>SNASDSASKDIITMKGDTIRVSDLYKEAKQFPSQPTNTLLQNLTFDKIFTKDFGKEVTDKDVSKKVKSIKDQYGSQFSSALQQQGLTEASFTPYMRTQMLEQAAIDHEIKETQYTDANLKKAWESYHPDVTAYVVSETSKDAATKALDAAKKDDAGKASFEKTNAESKVTFNSTSTSVPTEVQTAAFKLKNGEFSDVIESTSSSTGATSYYIVEM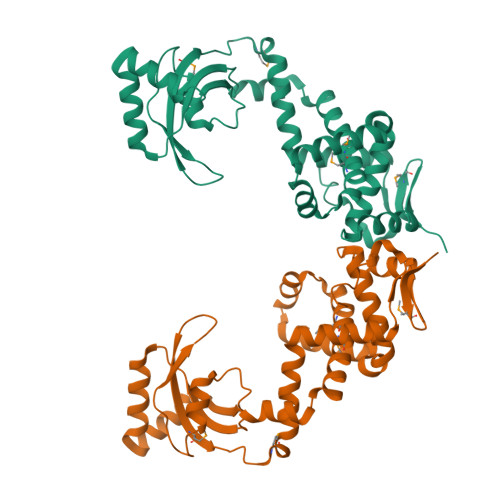VKTSEKGTDMNKYKKELQNVIKTEKEQDTTFVSGVIAKYLKKNNVTVKESAFASLFSQFTQTSSSSSSK[4x]> MSKAAKAKKNVPVVSKLEADARKAAEGVNDNESEEFKKAMRKEARALVEQFNEEKKLLAFYQQERQKINYNWIIAKKELEDKKSELINKEREIQDLQENHFMTLNVYKQKIKHLLFQNQDQQSELKKDVEVTLKQLEDQHRIKSRELKTDVRSLKVTKKEQEISQQDYLFALKSEHDKQMTLMRQDYERQVNDIKRKYDLKMQNLTKEMEEARAAMIKQLEDNKNQKIAEIIKEHTQKYNDIKNYYSEITATNLDYRKTLKNEIKELQTKDEEYKKTLQQTEKGYKELNEPLQALGIEIIQLKKQDEEQEAIIKEKEELKQKIDNQERLFRKLEYEYEVKLQQFQYLERERNALYAKFNQTVFEIHQKSGLENLILEKKVTNLREDLEIKDLQIHQVLTAANIDPNSVGSINKS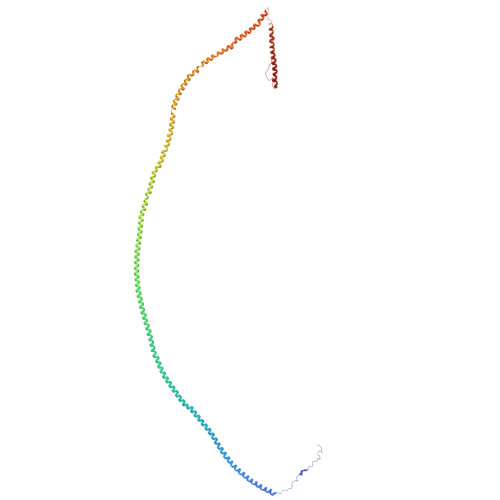LEEVESLKNELISELQAQLKQIRKAHSHMVKAYEGKLSEFVIPVEELGFDPLVPTNTD> MTLNTIALELVPPNSDGPDGGREQAVEDARKVLRCAAETGLAGRIGHVMIPGMIEEDPDRPIPMKPKMDVLDFWTIIRPELPGIRGLCTQVTAFLDEPALRRRLGDL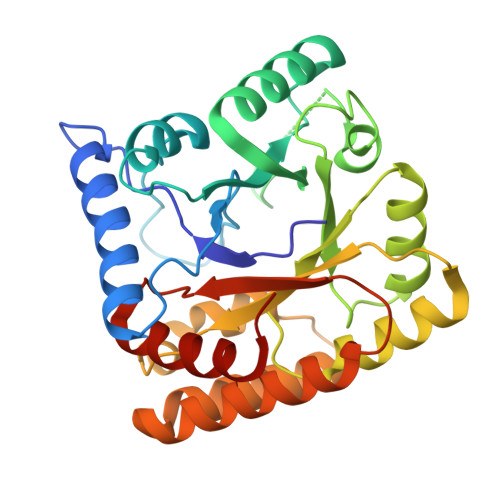SAAGFDGIAFVGVPRTMNDGEGHGVAPTDALSMFADLVPNRGAILIPTRDGEQGRFEFKCERGATYGMTQLLYSDAIVGFLREFARRTDHRPEILLSFGFVPKLEAKVGLINWLIQDPGNPAVAAEQEFVRRLAGLEPADKRKLMVDLYKRVIDGVADLGFPLSVHLEATYGVSVPAFETFAEMLAYWSPGQG>[2x]APITAYAQQTRGLLGCIITSLTGRDKNQVEGEVQIVSTATQTFLATCINGV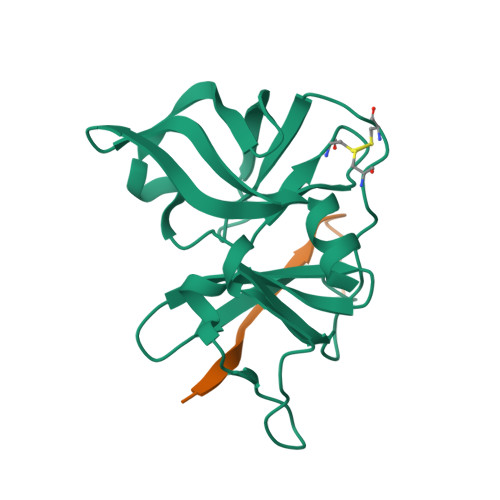CWTVYHGAGTRTIASPKGPVIQMYTNVDQDLVGWPAPQGSRSLTPCTCGSSDLYLVTRHADVIPVRRRGDSRGSLLSPRPISYLKGSSGGPLLCPAGHAVGLFRAAVCTRGVAKAVDFIPVENLETTMRS;>[2x]KGSVVIVGRIVLSGKPAIIPA>DSIIHIGAIFEENAAKDDRVFQLAVSDLSLNDDILQSEKITYSIKVIEANNPFQAVQEACDLMTQGILALVTSTGCASANALQSLTDAMHIPHLFVQRNPGGSPRTACHLNPSPDGEAYTLASRPPVRLNDVMLRLVTELRWQKFVMFYDSEYDIRGLQSFLDQASRLGLDVSLQKVDKNISHVFTSLFTTMKTEELNRYRDTLRRAILLLSPQGAHSFINEAVETNLASKDSHWVFVNEEISDPEILDLVHSALGRMTVVRQIFPSAKDNQKCMRNNHRISSLLCDPQEGYLQMLQISNLYLYDSVLMLANAFHRKLEDRKWHSMASLNCIRKSTKPWNGGRSMLDTIKKGHITGLTGVMEFREDSSNPYVQFEILGTTYSETFGKDMRKLATWDSEKGLNGSLQERPMGSRLQGLTLKVVTVLEEPFVMVAENILGQPKRYKGFSIDVLDALAKALGFKYEIYQAPDGRYGHQLHNTSWNGMIGELISKRADLAISAITITPERESVVDFSKRYMDYSVGILIKKPEEKISIFSLFAPFDFAVWACIAAAIPVVGVLIFVL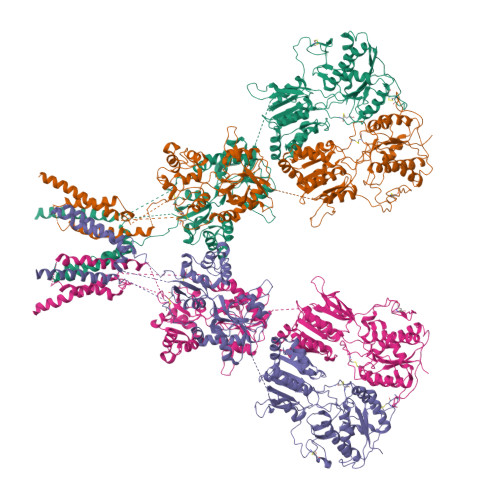NRIQAVRSQSATQPRPSASATLHSAIWIVYGAFVQQGGESSVNSVAMRIVMGSWWLFTLIVCSSYTANLAAFLTVSRMDSPVRTFQDLSKQLEMSYGTVRDSAVYEYFRAKGTNPLEQDSTFAELWRTISKNGGADNCVSNPSEGIRKAKKGNYAFLWDVAVVEYAALTDDDCSVTVIGNSISSKGYGIALQHGSPYRDLFSQRILELQDTGDLDVLKQKWWPHTGRCDLTSHSSAQTDGKSLKLHSFAGVFCILAIGLLLACLVAALELWWNSNRCHQETPKEDKEVGLVPR[4x]> MAQFAFESDLHSLLQLDAPIPNAPPARWQRKAKEAAGPAPSPMRAANRSHSAGRTPGRTPGKSSSKVQTTPSKPGGDRYIPHRSAAQMEVASFLLSKENQPENSQTPTK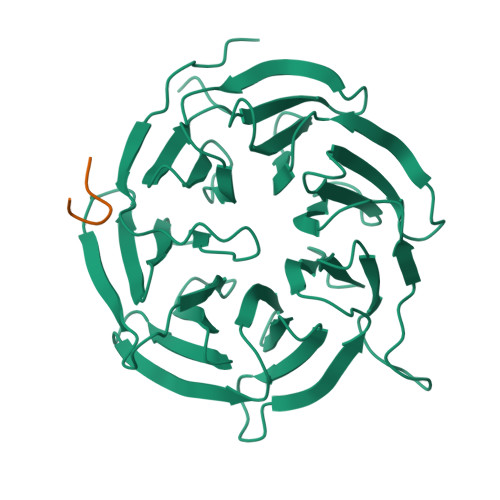KEHQKAWALNLNGFDVEEAKILRLSGKPQNAPEGYQNRLKVLYSQKATPGSSRKTCRYIPSLPDRILDAPEIRNDYYLNLVDWSSGNVLAVALDNSVYLWSASSGDILQLLQMEQPGEYISSVAWIKEGNYLAVGTSSAEVQLWDVQQQKRLRNMTSHSARVGSLSWNSYILSSGSRSGHIHHHDVRVAEHHVATLSGHSQEVCGLRWAPDGRHLASGGNDNLVNVWPSAPGEGGWVPLQTFTQHQGAVKAVAWCPWQSNVLATGGGTSDRHIRIWNVCSGACLSAVDAHSQVCSILWSPHYKELISGHGFAQNQLVIWKYPTMAKVAELKGHTSRVLSLTMSPDGATVASAAADETLRLWRCFELDPARRREREKASAAKSSLIHQGIR;> RAPXSDITN> MAKKTSSKGKLPPGPTPLPIIGNMLQIDVKDICKSFTNFSKVYGPVFTVYFGMNPIVVFHGYEAVKEALIDNGEEFSGRGNSPISQRITKGLGIISSNGKRWKEIRRFSLTTLRNFGMGKRSIEDRVQEEAHCLVEELRKTKASPCDPTFILGCAPCNVICSVVFQKRFDYKDQNFLTLMKRFNENFRILNSPWIQVCNNFPLLIDCFPGTHNKVLKNVALTRSYIREKVKEHQASLDVNNPRDFIDCFLIKMEQEKDNQKSEFNIENLVGTVADLFVAGTETTSTTLRYGLLLLLKHPEVTAKVQEEIDHVIGRHRSPCMQDRSHMPYTDAVVHEIQRYSDLVPTGVPHAVTTDTKFRNYLIPKGTTIMALLTSVLHDDKEFPNPNIFDPGHFLDKNGNFKKSDYFMPFSAGKRI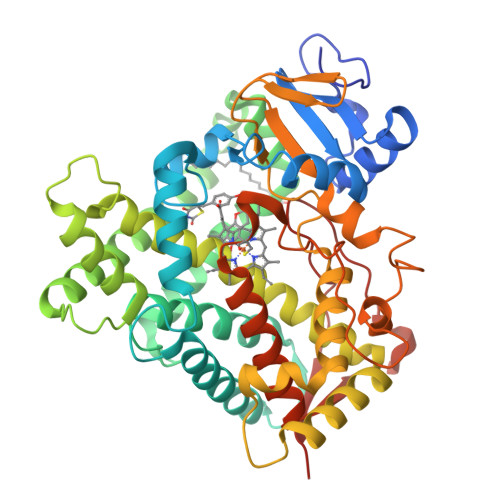CAGEGLARMELFLFLTTILQNFNLKSVDDLKNLNTTAVTKGIVSLPPSYQICFIPVHHHH>VADPRPDPDELARRAAQVIADRTGIGEHDVAVVLGSGWLPAVAALGSPTTVLPQAELPGFVPPTAAGHAGELLSVPIGAHRVLVLAGRIHAYEGHDLRYVVHPVRAARAAGAQIMVLTNAAGGLRADLQVGQPVLISDHLNLTARSPLVGGEFVDLTDAYSPRLRELARQSDPQLAEGVYAGLPGPHYETPAEIRMLQTLGADLVGMSTVHETIAARAAGAEVLGVSLVTNLAAGITGEPLSHAEVLAAGAASATRMGALLADVIARF[3x]

Purine nucleoside phosphorylases (PNPs, EC 2.4.2.1) are cytosolic enzymes involved in the purine salvage pathway metabolism in most organisms. The enzyme degrades (2′-deoxy)nucleosides based on 6-oxopurines to the corresponding purine bases and (2-deoxy)ribose-1-phosphate. Purine nucleoside phosphorylase (PNP) is a well-known molecular target with potential therapeutic applications in the treatment of T-cell malignancies and/or bacterial/parasitic infections. The results are supported by a crystallographic study of eight enzyme-inhibitor complexes and by ADMET profiling in vitro and in vivo.

To obtain information on the binding pose and interacting residues, crystal structures of recombinant MtPNP in complex with inhibitors 18c, 45b, and 45q were determined and refined to high resolution. Inhibitors 18c, 45b, and 45q bind to the active site of MtPNP through eight direct and three water-mediated hydrogen bonds. Compounds 45b and 45q have different substitutions at the central phenyl moiety. Substitution by bromine at position C4 leads to changes in the orientation of the phenyl moiety as well as the shift of helix (same as in human PNP) to avoid sterically clashing with a side chain of His243. These structural changes do not affect inhibitor affinity toward MtPNP since the IC50 values for each inhibitor are similar, leading to a conclusion that the active site is flexible and the movement of the helix allows the protein to accommodate inhibitors with different substitutions at positions C4 and C5 of the central phenyl moiety. Crystals of MtPNP in complex with 45b and 45q were obtained using the EasyXtal 15-Well Tool, hanging drop plates with reservoir volumes of 500 μL and 2 μL drops with protein:reservoir ratio 1:1. Crystals of MtPNP/45q were obtained using the reservoir containing 25 mM magnesium chloride, 100 mM TRIS pH 7.5, and 25% w/v PEG4000. Plate crystal dimensions 400 × 150 × 10 μm grew in 3 weeks.> MQAIKESYAFAVLGEPRYAFNFNHFDYVNPAAPKGGQITLSALGTFDNFNRYALRGNPGARTEQLYDTLFTTSDDEPGSYYPLIAESARYADDYSWVEVAINPRARFHDGSPITARDVEFTFQKFMTEGVPQFRLVYKGTTVKAIAPLTVRIELAKPGKEDMLSLFSLPVFPEKYWKDHKLSDPLATPPLASGPYRVTSWKMGQNIVYSRVKDYWAA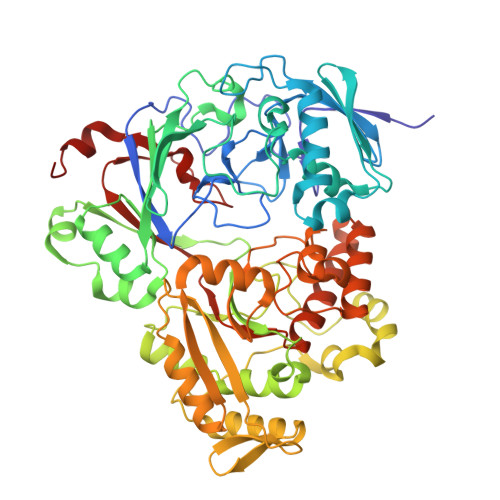NLPVNRGRWNFDTIRYDYYLDDNVAFEAFKAGAFDLRMENDAKNWATRYTGKNFDKKYIIKDEQKNESAQDTRWLAFNIQRPVFSDRRVREAITLAFDFEWMNKALFYNAWSRTNSYFQNTEYAARNYPDAAELVLLAPMKKDLPSEVFTQIYQPPVSKGDGYDRDNLLKADKLLNEAGWVLKGQQRVNATTGQPLSFELLLPASSNSQWVLPFQHSLQRLGINMDIRKVDNSQITNRMRSRDYDMMPRVWRAMPWPSSDLQISWSSEYINSTYNAPGVQSPVIDSLINQIIAAQGNKEKLLPLGRALDRVLTWNYYMLPMWYMAEDRLAWWDKFSQPAVRPIYSLGIDTWWYDVNKAAKLPS>DSELQLVEQRIRSFPDFPTPGVVFRDISPVLKDPASFRAAIGLLARHLKATHGGRIDYIAGLDSRGFLFGPSLAQELGLGCVLIRKRGKLPGPTLWASYSLEFGKAELEIQK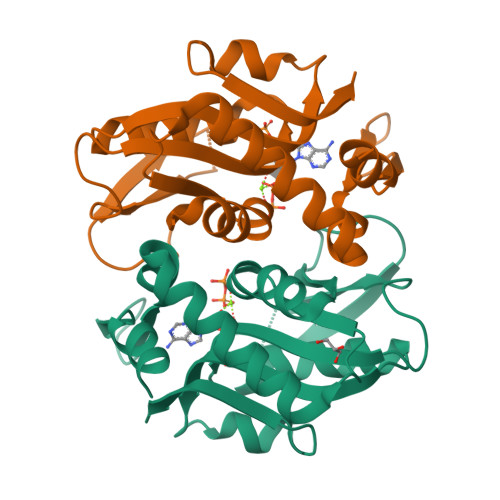DALEPGQRVVVVDDLLATGGTMNAACELLGRLQAEVLECVSLVELTSLKGREKLAPVPFFSLLQYE[2x]>[4x]MEVDPRLYFENRSKFIQDQKDKGINPYPHKFERTISIPEFIEKYKDLGNGEHLEDTILNITGRIMRVSASGQKLRFFDLVGDGEKIQVLANYSFHNHEKGNFAECYDKI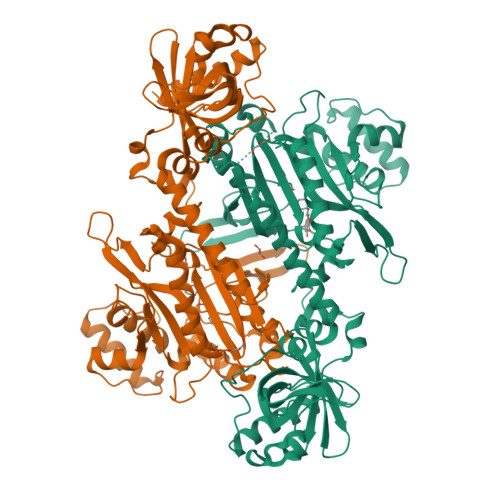RRGDIVGIVGFPGKSKKGELSIFPKETILLSACLHMLPMKYGLKDTEIRYRQRYLDLLINESSRHTFVTRTKIINFLRNFLNERGFFEVETPMMNLIAGGANARPFITHHNDLDLDLYLRIATELPLKMLIVGGIDKVYEIGKVFRNEGIDNTHNPEFTSCEFYWAYADYNDLIKWSEDFFSQLVYHLFGTYKISYNKDGPENQPIEIDFTPPYPKVSIVEEIEKVTNTILEQPFDSNETIEKMINIIKEHKIELPNPPTAAKLLDQLASHFIENKYNDKPFFIVEHPQIMSPLAKYHRTKPGLTERLEMFICGKEVLNAYTELNDPFKQKECFKLQQKDREKGDTEAAQLDSAFCTSLEYGLPPTGGLGLGIDRITMFLTNKNSIKDVILFPTMRPANGGHHHHHH>MTAENSATPDYRRNVGAVADALLAHPGPIVVLSHENPDGDALGSVLGLSRALRTLGKTVLAPMTVPHYLSFLPQPGELTAPLESWPQGALAAVLDVDNNDPVRVAGADLTQFDGPVVNVDHHGTNLRRADAGVVDPSKPAAAMMVADVIDALGAPWSEAVATPLMLGLNTDTGNFAFDSVSAETFECAARLRAHGARIGWLNDQMRQNPQSYYLLLREVLGKLEFLHGGRVVQTRVDEEMLARAGATWEQVENYVSMLRNAEGAQLAVMAKDYGDRVKFSLRSRGPVSAQNIAVALGGGGHVPAAGATVISSYAEARARLDAAIEAELARVDAQATAE[3x]

Members of the most radioresistant bacteria genus, Deinococcus, possess two DHH/DHHA1 family proteins, RecJ and RecJ-like. In contrast, DrRecJ-like only harbors a DHH and a DHHA1 domain and its biochemical features and biological functions have not been studied. DrRecJ-like exhibits a preferred catalytic activity towards short single-stranded RNA/DNA oligos and c-di-AMP.

Moreover, a crystal structure of DrRecJ-like, with Mg2+ bound in an open conformation at a resolution of 1.97 Å, has been resolved. The full-length DrRecJ-like protein, free from any substrate or product, was successfully crystallized in space group C121. The refined DrRecJ-like structure comprises three protomers in the asymmetric unit, with two of the protomers forming a dimer and the remaining protomer forming a dimer with a symmetrical protomer from a neighboring molecule. The crystallization condition used in our study contained MgSO4, and we observed two Mg2+ ions bound at the active site. Two catalytic metal ions (Mg2+) coordinated by conserved histidine and aspartate residues (H34, D38, D40, D95, H121, and D171) were observed in the catalytic core. The second ‘H’ of the DHH motif (H122) was not directly bound to the catalytic metal ions. Although our crystals were soaked with the putative product, AMP, before being frozen, there was no AMP density in the map. This suggests that the open state of the DrRecJ-like protein has very weak affinity for its cleavage products. Like other structurally characterized NrnA homologs, each protomer of DrRecJ-like consists of a conserved DHH domain, in which five stranded β-sheets (21345, ↑↑↑↑↑) are sandwiched between a series of α-helices, and a conserved DHHA1 domain, in which six stranded β-sheets (123465, ↓↑↑↓↑↓) are sandwiched between a series of α-helices. According to the structural data, dimerization of DrRecJ-like is mediated by hydrophobic interactions between several α-helices (the α7 and α8 on the DHH domain, and the α10 and α12 on the DHHA1 domain) of protomers.> IVGGYTCGANTVPYQVSLNSGYHFCGGSLINSQWVVSAAHCYKSGIQVRLGEDNINVVEGNEQFISASKSIVHPSYNSNTLNNDIMLIKLKSAASLNSRVA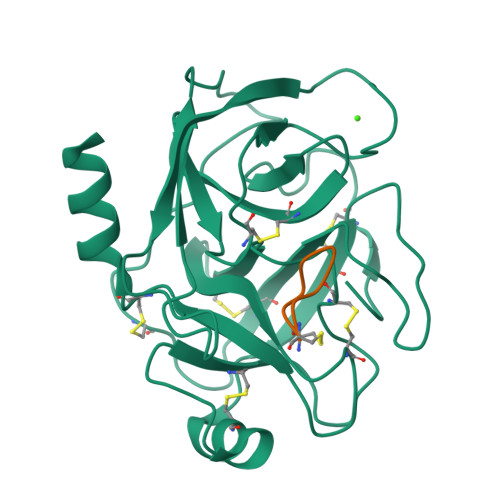SISLPTSCASAGTQCLISGWGNTKSSGTSYPDVLKCLKAPILSDSSCKSAYPGQITSNMFCAGYLEGGKDSCQGDSGGPVVCSGKLQGIVSWGSGCAQKNKPGVYTKVCNYVSWIKQTIASN;> EPCCDSCRCTKSIPPECHCANI>MASQSSVAVISSAAARGESFPDSKKPIGSVRFQQPLRLSFSYCKSGNMSSRICAMAKPNDAETLSSSVDMSLSPRVQSLKPSKTMVITDLAATLVQSGVPVIRLAAGEPDFDTPKVVAEAGINAIREGFTRYTLNAGITELREAICRKLKEENGLSYAPDQILVSNGAKQSLLQAVLAVCSPGDEVIIPAPYWVSYTEQARLADATPVVIPTKISNNFLLDPKDLESKLTEKSRLLILCSPSNPTGSVYPKSLLEEIARIIAKHPRLLVLSDEIYEHIIYAPATHTSFASLPDMYERTLTVNGFSKAFAMTGWRLGYLAGPKHIVAACSK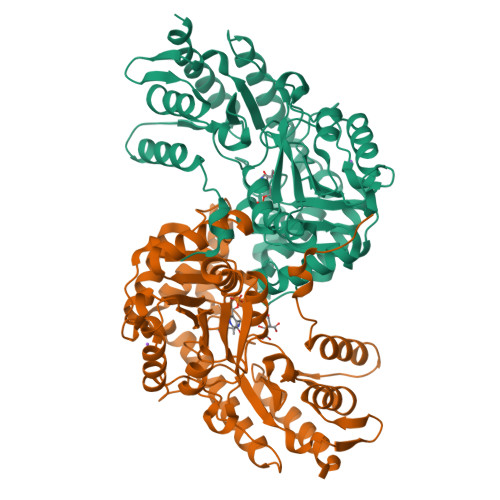LQGQVSSGASSIAQKAGVAALGLGKAGGETVAEMVKAYRERRDFLVKSLGDIKGVKISEPQGAFYLFIDFSAYYGSEAEGFGLINDSSSLALYFLDKFQVAMVPGDAFGDDSCIRISYATSLDVLQAAVEKIRKALEPLRATVSV[4x]> MMFGRFTERAQKVLALAQEEALRLGHNNIGTEHILLGLVREGEGIAAKALQALGLGSEKIQKEVESLIGRGQEMSQTIHYTPRAKKVIELSMDEARKLGHSYVGTEHILLGLIREGEGVAARVLNNLGVSLNKARQQVLQLLGSNETGSSAAGTNSNANTPTLDSLARDLTAIAKEDSLDPVIGRSKEIQRVIEVLSRRTKNNPVLIGEPGVGKTAIAEGLAQQIINNEVPEILRDKRVMTLDMGTVVAGTKYRGEFEDRLKKVMDEIRQAGNIILFIDELHTLIGAGGAEGAIDASNILKPSLARGELQCIGATTLDEYRKYIEKDAALERRFQPIQVDQPSVDESIQILQGLRDRYEAHHRVSITDDAIEAAVKLSDRYISDRFLPDKAIDLIDEAGSKVRLRSFTTPPNLKELEQKLDEVRKEKDAAVQSQEFEKAASLRDTEQRLREQVEDTKKSWKEKQGQENSEVTVDDIAMVVSSWTGVPVSKI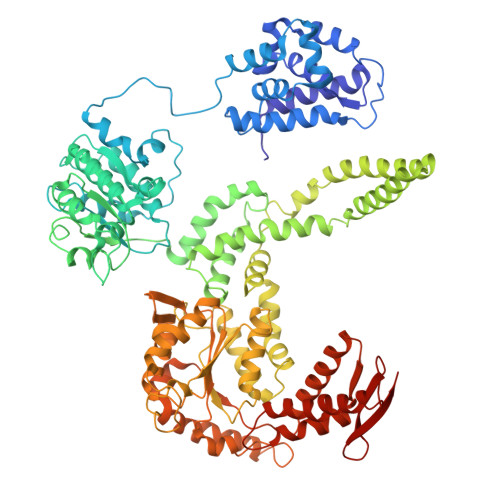AQTETDKLLNMENILHSRVIGQDEAVVAVAKAVRRARAGLKDPKRPIGSFIFLGPTGVGKTELARALAESIFGDEESMIRIDMSEYMEKHSTSRLVGSPPGYVGYDEGGQLTEKVRRKPYSVVLLDAIEKAHPDVFNILLQVLEDGRLTDSKGRTVDFRNTILIMTSNVGASELKRNKYVGFNVQDETQNHKDMKDKVMGELKRAFRPEFINRIDEIIVFHSLEKKHLTEIVSLMSDQLTKRLKEQDLSIELTDAAKAKVAEEGVDLEYGARPLRRAIQKHVEDRLSEELLRGNIHKGQHIVLDVEDGEFVVKTTAKTN>[4x]GSMLTGVIEGFYGRDWRRDERATVMDWIAAAGMNTYIYGPKDDVHVRARWRVPYDAAGLARLTELRDAAAARGMVFYVSLAPCLDVTYSDPQDRAALLARVDQLARAGLRNLVLLFDDIPSVLPEADRHRFDSFAEAQADLS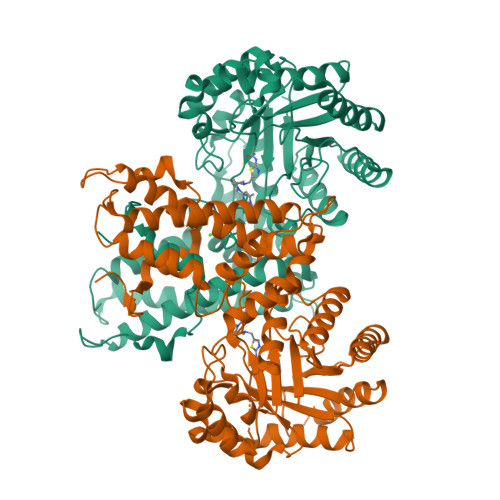NMVLRHLRGAGHVVFCPTEYCGRMAGGDPRGSAYLQRLGSTLDPAIDIFWTGPEIVSEEIVAAHLAAVGEVLRRRPVIWDNFHANDYDIRRVFAGPLGGRSRDILPLVAGWITNPNNEAEANFPAIHTTGAYLADPDYAPERAIAAAVAAWQPRFRLAFGDGAVPSDLVALLCDLFWQPFALGPETTRILSALRAALTVPRPDPSDPAWRAALEDLRDLKRRINKLFTLMTEIENRDLFHTFHNYLWEAQEEVGHLVAYCDWLDEAPPPGAVFPATDRIHNFYRRGFGVAVQDILQRDRQGRYHHGV> MKKLQIAVGIIRNENNEIFITRRAADA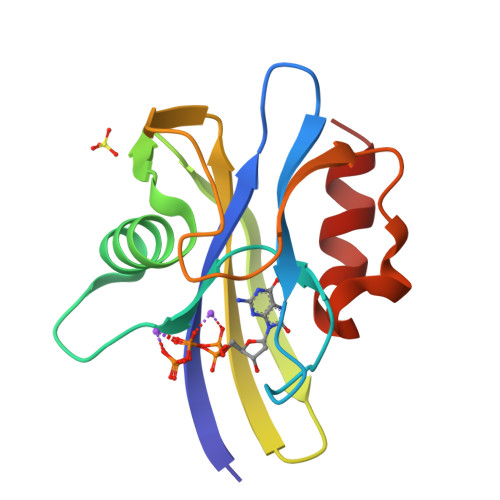HMANKLEFPGGKIEMGETPEQAVVRELQEEVGITPQHFSLFEKLEYEFPDRHITLWFWLVERWEGEPWGKEGQPGEWMSLVGLNADDFPPANEPVIAKLKRL>[2x]GETTDTKREEQEIEEKKAQEESKIEDVDKILNDILSISSECIQPDELRVKLLLKRKLICYDGFEPSGRMHIAQGLLKSIIVNKLTSNGCTFIFWIADW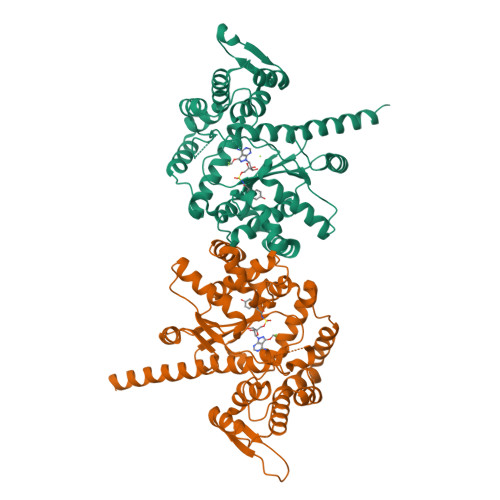FAHLNNKMSGDLKKIKKVGSYFIEVWKSCGMNMENVQFLWASEEINKKPNEYWSLVLDISRSFNINRMKRCLKIMGRSEGEENYCSQILYPCMQCADIFFLNVDICQLGIDQRKVNMLAREYCDIKKIKKKPVILCHGMLPGLLEGQEKMSKSDENSAIFMDDSESDVNRKIKKAYCPPNVIENNPIYAYAKSIIFPSYNEFNLVRKEKNGGDKTYYTLQELEHDYVNGFIHPLDLKDNVAMYINKLLQPVRDHFQNNIEAKNLLNEIKKYKVTK In Gram-negative bacteria, Fe3+-siderophore complexes are recognised at the bacterial cell surface by highly selective outer-membrane TonB-dependent transporters (TBDTs). These transporters bind the Fe3+-siderophore complex and translocate it into the periplasm. The structures of pyoverdine, pyochelin, citrate and ferrichrome iron complexes bound to their respective transporters FpvA, FptA, FecA and FhuA showed that the ferric-siderophore complexes were bound inside the barrel adjacent to the plug domain, a position thought to be poised for translocation. Pseudomonas aeruginosa, a serious opportunistic pathogen, does not make enterobactin but does possess a TBTD outer-membrane protein PfeA, related to FepA, that binds and translocates Fe3+-enterobactin into the periplasm. PfeA has the same two domains (22-stranded β-barrel and N-terminal plug) common to the TBDTs.

Azotochelin and protochelin are two siderophores produced by Azotobacter vinelandii, an environmental Gram-negative bacterium. Fe3+-enterobactin, Fe3+-azotochelin and Fe3+-protochelin coelute with PfeA on a size-exclusion column suggesting each of them are bound by PfeA. Crystal structures show that these two molecules bind in the same location as enterobactin (with less than 0.5 Å shift between the relative position of the iron atoms) and two of the catecholate rings occupy the same positions as rings II and III of enterobactin. Hydrogen bonds between the catecholates and Ser479, Gly325 and Arg480 are conserved. In the azotochelin complex, a molecule of ethylene glycol from the crystallisation solution completes the coordination shell of the iron, and this molecule interacts with Gln482. The stacking interaction between Arg480 and catecholate II has been conserved. However, the side chain of Gln482 is unable to form a hydrogen bond with the aliphatic backbone of azotochelin, and is slightly displaced. The carboxylate group of the backbone is pointing towards the surface of the protein in the vicinity of Arg480 and Lys218. The positioning of the three rings is clearly important in making the optimum interactions with the protein, indicating there are constraints on the linkage geometry. It is, however, worth noting that the connection of the rings tolerates the addition of at least one extra carbon, seen with protochelin and that a molecule with only two rings (azotochelin) can be efficiently bound.

> GAMAGQGDGSVIELGEQTVVATAQEETKQAPGVSIITAEDIAKRPPSNDLSQIIRTMPGVNLTGNSSSGQRGNNRQIDIRGMGPENTLILVDGKPVSSRNSVRYGWRGERDSRGDTNWVPADQVERIEVIRGPAAARYGNGAAGGVVNIITKQAGAETHGNLSVYSNFPQHKAEGASERMSFGLNGPLTENLSYRVYGNIAKTDSDDWDINAGHESNRTGKQAGTLPAGREGVRNKDIDGLLSWRLTPEQTLEFEAGFSRQGNIYTGDTQNTNSNNYVKQMLGHETNRMYRETYSVTHRGEWDFGSSLAYLQYEKTRNSRINEGLAGGTEGIFDPNNAGFYTATLRDLTAHGEVNLPLHLGYEQTLTLGSEWTEQKLDDPSSNTQNTEEGGSIPGLAGKNRSSSSSARIFSLFAEDNIELMPGTMLTPGLRWDHHDIVGDNWSPSLNLSHALTERVTLKAGIARAYKAPNLYQLNPDYLLYSRGQGCYGQSTSCYLRGNDGLKAETSVNKELGIEYSHDGLVAGLTYFRNDYKNKIESGLSPVDHASGGKGDYANAAIYQWENVPKAVVEGLEGTLTLPLADGLKWSNNLTYMLQSKNKETGDVLSVTPRYTLNSMLDWQATDDLSLQATVTWYGKQKPKKYDYHGDRVTGSANDQLSPYAIAGLGGTYRLSKNLSLGAGVDNLFDKRLFRAGNAQGVVGIDGAGAATYNEPGRTFYTSLTASF> 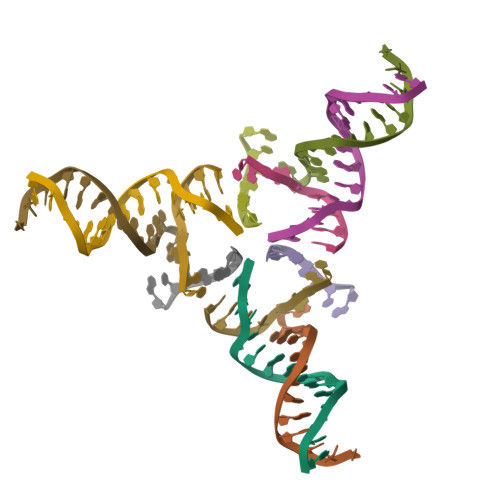ACGGACAGCAGTGCA;> CACACCGT;> CTGCACTGCTGTG;> GCTGTG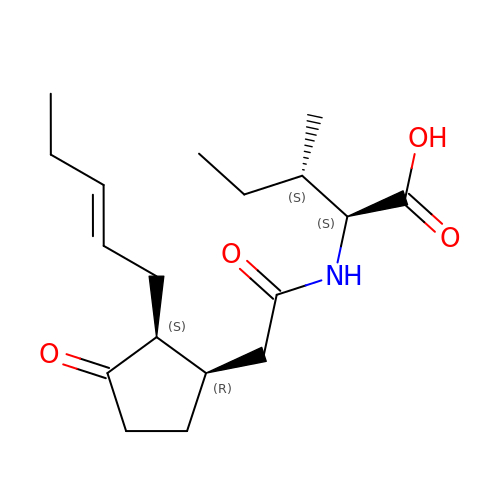N-({(1R,2S)-3-oxo-2-[(2Z)-pent-2-en-1-yl]cyclopentyl}acetyl)-L-isoleucine | C18 H29 N O4 | IBZYPBGPOGJMBF-QPERPISQSA-N5-[2-(4-chlorophenoxy)phenyl]-2-methyl-1H-pyrrole-3-carboxamide | C18 H15 Cl 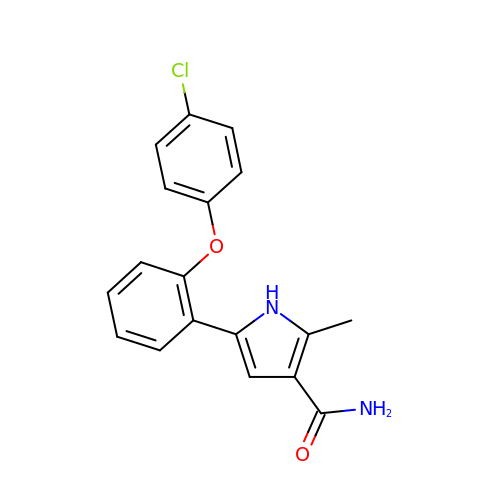N2 O2 | VYHWNVJEEBHTKR-UHFFFAOYSA-N> SFRDNLKVYIESPESYKNVIYYDDDVVLVRDMFPKSKMHLLLMTRDPHLTHVHPLEIMMKHRS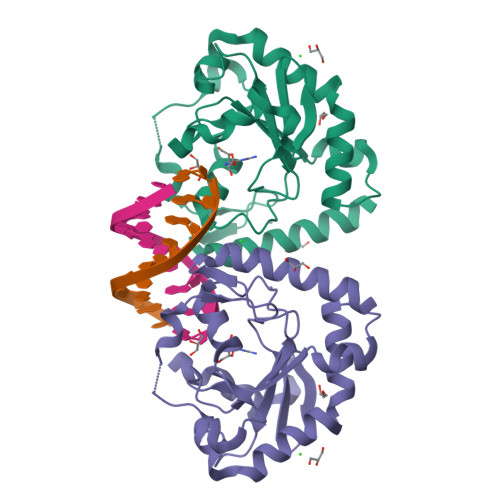LVEKLVSYVQGDLSGLIFDEARNCLSQQLTNEALCNYIKVGFHAGPSMNNLHLHIMTLDHVSPSLKNSAHYISFTSPFFVKIDTPTSNLPTRGTLTSLFQEDLKCWRCGETFGRHFTKLKAHLQEEYDDWLDKSVSM1,1'-HEXANE-1,6-DIYLBIS(1H-IMIDAZOLE) | C12 H18 N4 | 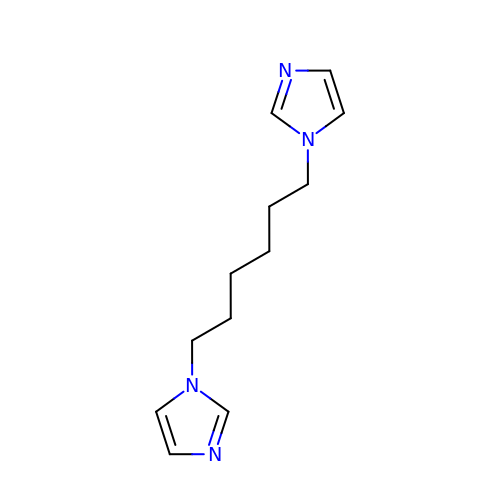CHRPUSCNMSNSKL-UHFFFAOYSA-N> GPLGSGQYKDNIRHGVCWIYYPDGGSLVGEVNEDGEMTGEKIAYVYPDERTALYGKFIDGEMIEGKLATLMSTEEGRPHFELMPGNSVYHFDKSTSSCISTNALLPDPYESERVYVAESLISSAGEGLFSKVAVGPNTVMSFYNGVRITHQEVD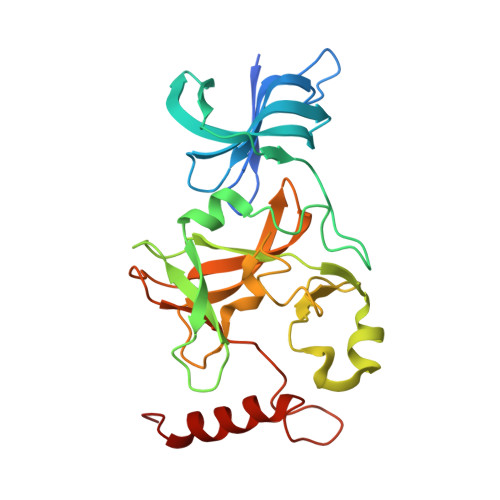SRDWALNGNTLSLDEETVIDVPEPYNHVSKYCASLGHKANHSFTPNCIYDMFVHPRFGPIKCIRTLRAVEADEELTVAYGYDHSPPGKSGPEAPEWYQVELKAFQATQQK> MQTLKELIASNPDDLTTELKRAFRPLTPHIAIDGNELDALTILVNLTDKTDDQKDLLDRAKCKQKLRDEKWWASCINCVNYRQSHNPKFPDIRSEGVIRTQALGELPSFLLSSSKIPPYHWSYSHDSKYVNKSAFLTNEFCWDGEISCLGELLKDADHPLWNTLKKLGCSQKTCKAMAKQLADITLTTINVTLAPNYLTQISLPDSDTSYISLSPVASLSMQSHFHQRLQDENRHSAITRFSRTTNMGVTAMTCGGAFRMLKSGAKFSSPPHHRLNSKRSWLTSEHVQSLKQYQRLNKSLIPENSRIALRRKYKIELQNMVRSWFAMQDHTLDSNILIQHLNHDLSYLGATKRFAYDPAMTKLFTELLKRELSNSINNGEQHTNGSFLVLPNIRVCGATALSSPVTVGIPSLTAFFGFVHAFERNINRTTSSFRVESFAICVHQLHVEKRGLTAEFVEKGDGTISAPATRDDWQCDVVFSLI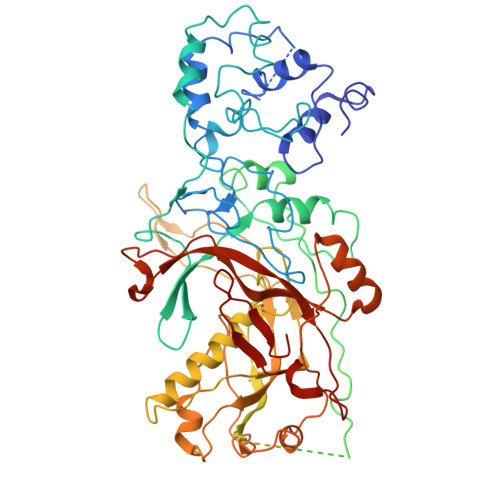LNTNFAQHIDQDTLVTSLPKRLARGSAKIAIDDFKHINSFSTLETAIESLPIEAGRWLSLYAQSNNNLSDLLAAMTEDHQLMASCVGYHLLEEPKDKPNSLRGYKHAIAECIIGLINSITFSSETDPNTIFWSLKNYQNYLVVQPRSINDETTDKSSL> MEIGVVGKPNVGKSTFFSAATLVDVEIANYPFTTIEANVGVTYAITDHPCKELGCSPNPQNYEYRNGLALIPVKMVDVAGLVPGAHEGRGLGNKFLDDLRMASALIHVVDATGKTDPEGQPTDYHDPVEDIEFLEREIDYWIYGILS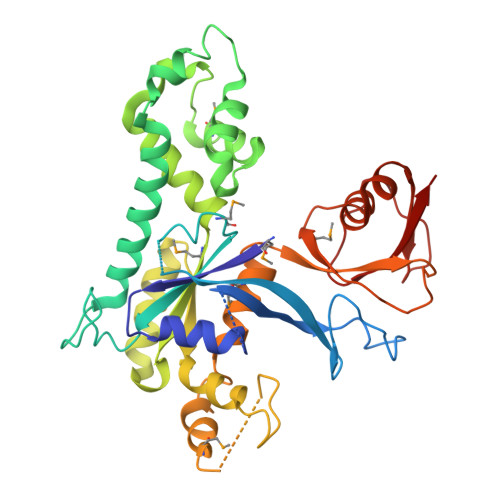KGWDKFAKRIKLQKIKLESAIAEHLSGIGVNENDVWEAMHKLNLPEDPTKWSQDDLLAFASEIRRVNKPMVIAANKADAASDEQIKRLVREEEKRGYIVIPTSAAAELTLRKAAKAGFIEYIPGASEFKVLRDMSEKQKRALMVIKEKVLDRFGSTGVQEVINRVVFDLLKLIPVYPVHDENKLTDQFGNVLPHVFLMKKGSTPRDLAFKVHTDLGKGFLYAINARTKRRVGEDYELQFNDIVKIVSVTR> MVRIIVKNVSKVFKKGKVVALDNVNINIENGERFGILGPSGAGKTTFMRIIAGLDVPSTGELYFDDRLVASNGKLIVPPEDRKIGMVFQTWALYPNLTAFENIAFPLTNMKMSKEEIRKRVEEVAKILDIHHVLNHFPRELSGAQQQRVALARALVKDPSLLLLDEPFSNLDARMRDSARA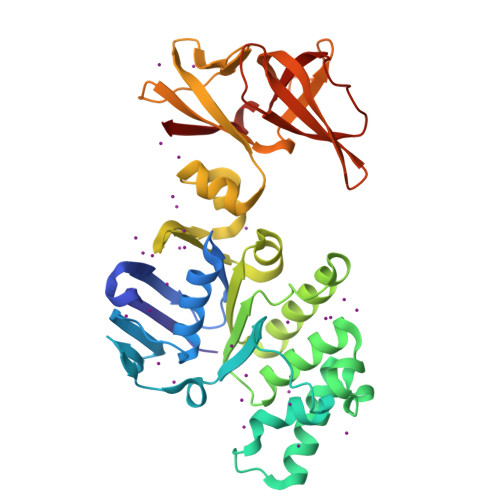LVKEVQSRLGVTLLVVSHDPADIFAIADRVGVLVKGKLVQVGKPEDLYDNPVSIQVASLIGEINELEGKVTNEGVVIGSLRFPVSVSSDRAIIGIRPEDVKLSKDVIKDDSWILVGKGKVKVIGYQGGLFRITITPLDSEEEIFTYSDHPIHSGEEVLVYVRKDKIKVFEKN> RAITVFSPDGRLFQVEYAR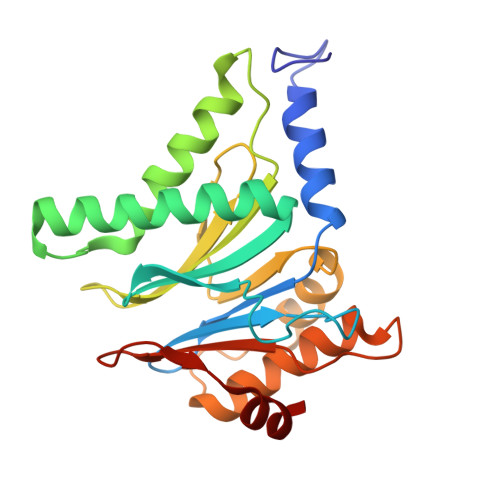EAVKKGSTALGMKFANGVLLISDKKVRSRLIEQNSIEAIQLIDDYVAAVTSGLVADARVLVDFARISAQQEKVTYGSLVNIENLVKRVADQMQQYTQYGGVRPYGVSLIFAGIDQIGPRLFDCDPAGTINEYKATAIGSGKDAVVSFLEREYKENLPEKEAVTLGIKALKSSLEEGEELKAPEIASITVGNKYRIYDQEEVKKFL> SPQPLEQIKLSESQLSGRVGMIEMDLASGRTLTAWRADERFPMMSTFKVVLCGAVLARVDAGDEQLERKIHYRQQDLVDYSPVSEKHLADGMTVGELCAAAITMSDNSAANLLLATVGGPAGLTAFLRQIGDNVTRLDRWA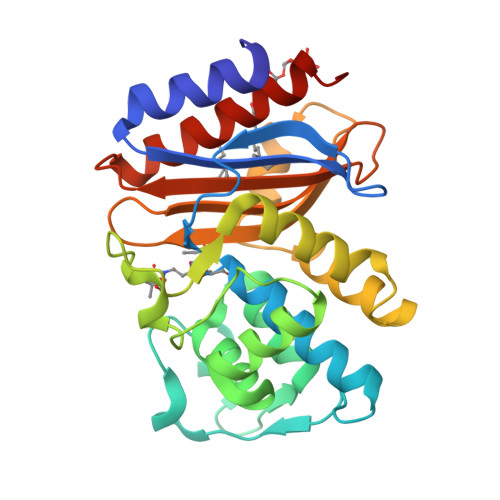TELNEALPGDARDTTTPASMAATLRKLLTSQRLSARSQRQLLQWMVDDRVAGPLIRSVLPAGWFIADKTGAGERGARGIVALLGPNNKAERIVVIYLRDTPASMAERNQQIAGIGAALIEHWQRLMNLV>[4x]MSEEISLSAEFIDRVKASVKPHWGKLGWVTYKRTYARWLPEKGRSENW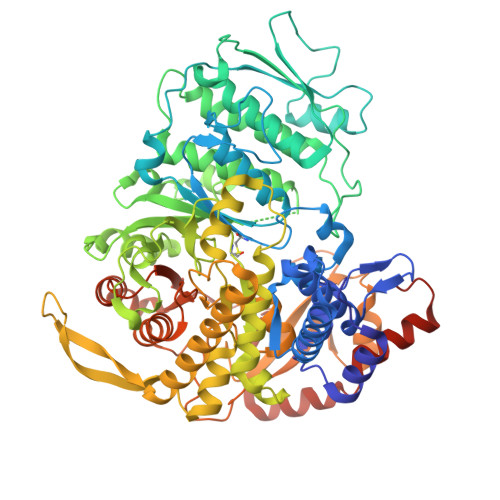DETVKRVVEGNINLDPRLQDSPSLELKQSLTEEAERLYKLIYGLGATPSGRNLWISGTDYQRRTGDSLNNCWFVAIRPQKYGDSKIVPSYLGKQEKAVSMPFSFLFDELMKGGGVGFSVARSNISQIPRVDFAIDLQLVVDETSESYDASVKVGAVGKNELVQDADSIYYRLPDTREGWVLANALLIDLHFAQTNPDRKQKLILDLSDIRPYGAEIHGFGGTASGPMPLISMLLDVNEVLNNKAGGRLTAVDAADICNLIGKAVVAGNVRRSAELALGSNDDQDFISMKQDQEKLMHHRWASNNSVAVDSAFSGYQPIAAGIRENGEPGIVNLDLSKNYGRIVDGYQAGIDGDVEGTNPCGEISLANGEPCNLFEVFPLIAEEQGWDLQEVFALAARYAKRVTFSPYDWEISREIIQKNRRIGISMSGIQDWLLTRLGNRVVTGFKDDFDPETHEAIKVPVYDKRAIKMVDQLYKAVVKADQDYSKTLGCNESIKHTTVKPSGTVAKLAGASEGMHFHYGAYLIQRIRFQDSDPLLPALKACGYRTEADIYTENTTCVEFPIKAVGADNPNFASAGTVSIAEQFATQAFLQTYWSDNAVSCTITFQDSEGDQVESLLRQYRFITKSTSLLPYFGGSLQQAPKEPIDKETYEKRSQEITGNVEEVFSQLNSDVKDLELVDQTDCEGGACPIK> MHLNPAEKEKLQIFLASELALKRKARGLKLNYPEAVAIITSFIMEGARDGKTVAMLMEEGKHVLTRDDVMEGVPEMIDDIQAEATFPDGTKLVTVHNPIS;> NYIVPGEYRVAEGEIEINAGREKTTIRVSNTGDRPIQVGSHIHFVEVNKELLFDRAEGIGRRLNIPSGTAARFEPGEEMEVELTELGGNREVFGIS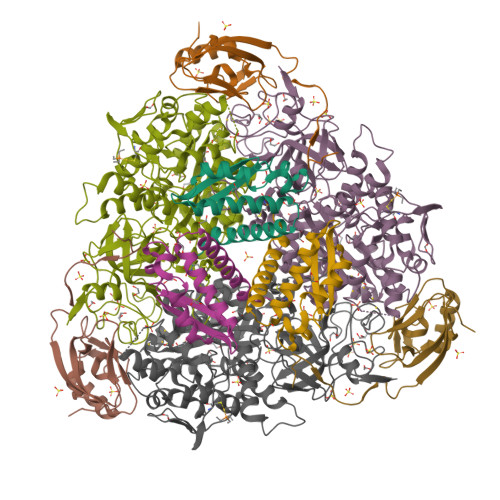DLTNGSVDNKELILQRAKELGYKGVE;> MKINRQQYAESYGPTVGDQVRLADTDLWIEVEKDYTTYGDEANFGGGKVLREGMGENGTYTRTENVLDLLLTNALILDYTGIYKADIGVKDGYIVGIGKGGNPDIMDGVTPNMIVGTATEVIAAEGKIVTAGGIDTHVHFINPDQVDVALANGITTLFGGGTGPAEGSKATTVTPGPWNIEKMLKSTEGLPINVGILGKGHGSSIAPIMEQIDAGAAGLKIHEDWGATPASIDRSLTVADEADVQVAIHSDTLNEAGFLEDTLRAINGRVIHSFHVEGAGGGHAPDIMAMAGHPNVLPSSTNPTRPFTVNTIDEHLDMLMVCHHLKQNIPEDVAFADSRIRPETIAAEDILHDLGIISMMSTDALAMGRAGEMVLRTWQTADKMKKQRGPLAEEKNGSDNFRAKRYVSKYTINPAIAQGIAHEVGSIEEGKFADLVLWEPKFFGVKADRVIKGGIIAYAQIGDPSASIPTPQPVMGRRMYGTVGDLIHDTNITFMSKSSIQQGVPAKLGLKRRIGTVKNCRNIGKKDMKWNDVTTDIDINPETYEVKVDGEVLTCEPVKELPMAQRYFLF> GPGGHMANFDFDVWRKKYMRWMNHKKSRVMDFFRRIDKDQDGKITRQEFIDGILAS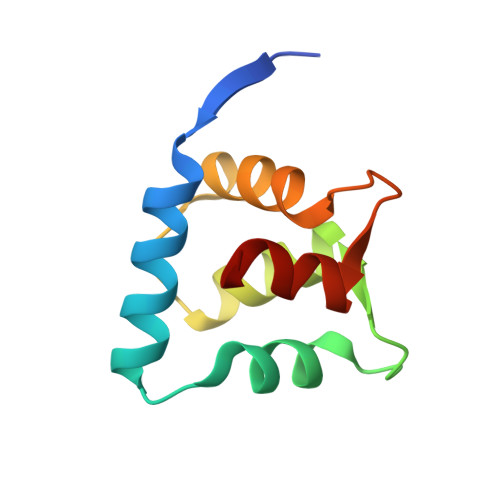KFPTTKLEMTAVADIFDRDGDGYIDYYEFVAALHP1,3-benzodioxol-5-ol | C7 H6 O3 | 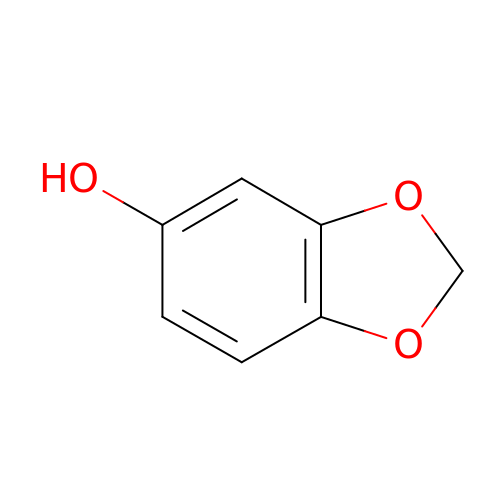LUSZGTFNYDARNI-UHFFFAOYSA-N> GPGSSEHKAKYENVTKDIFDLRDYYSGASKELKNVTGYRYSKGGKHYLIFDAHQAFTRIQIFGKDIERLKARKNPGLDIFVVKEAENRNGTVFSYGGVTKKNQGAYYDYLNAPKFVIKKEVDAGVYTHVKRHYIYKEEVSLKELDFKLRQYLIQNFDLYKKFPKDSKIKVIMKDGGYYTFELNKKL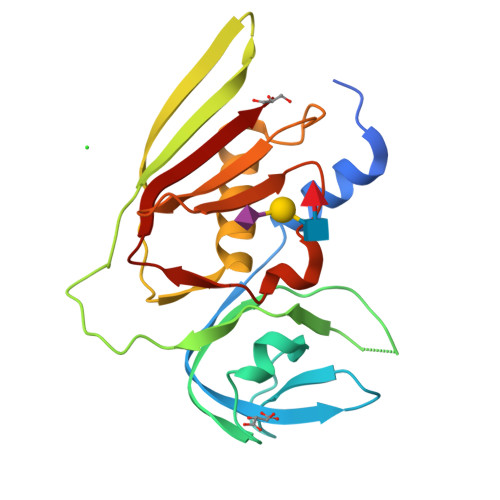QPHRMSDVIDGRNIEKMEANIR Conjugative type IV secretion systems (T4SS) mediate bacterial conjugation, a process that enables the unidirectional exchange of genetic materials between a donor and a recipient bacterial cell. Bacterial conjugation is the primary means by which antibiotic resistance genes spread among bacterial populations. The recent cryo-electron microscopy (cryo-EM) structure of the conjugative Type 4 Secretion System (T4SS) encoded by the plasmid R388 revealed that the remaining VirB proteins form a large assembly organised into four sub-complexes: the outer membrane core complex (OMCC), the stalk, the arches and the inner membrane complex (IMC). Previously, we solved the cryo-electron microscopy (cryo-EM) structure of a conjugative T4SS. In this article, based on additional data, we present a more complete T4SS cryo-EM structure than that published earlier.

Also, a fourth subunit of TrwG/VirB8 in the asymmetric unit of both the Arches (TrwG/VirB8peri) and the IMC (TrwG/VirB8tail) could be placed and built. Correspondingly, a fourth TrwG/VirB8tail is observed in the asymmetric unit of the IMC. Therefore, overall, there are 24 TrwG/VirB8 subunits in the T4SS. An intriguing feature of the T4SS structure solved previously was the paucity of interactions between the various sub-complexes (OMCC, Arches, Stalk and IMC). However, from the work presented here, VirB10 emerges as a crucial and unique element that ‘glues’ these distinct sub-complexes together. Another remarkable feature of VirB10 is that the T4SS include 16 copies of them, only 14 are used in the O-layer, potentially only 12 of them in the Arches, with only five of those involved in VirB6 binding and six involved in VirB4 ATPase contacts. One of the two VirB10Arches that we have observed runs very close to the VirB2 assembly site on VirB6 and we now know that VirB10IM in the IM obstructs the VirB2 recruitment site on VirB6, providing two other means by which VirB10 may be regulating pilus subunit recruitment and assembly. Finally, we observe a sequence of VirB10 (VirB10Cyto) that makes multiple contacts with the TrwK/VirB4 ATPase, thereby potentially providing another point of pilus biogenesis regulation.

>MKKLVMTAAVAAILGAASPVMAQGIPVFDGTRALDFVQQFARMKEQLDTAKDQLAEAQRMYEAVTGGRGLGDLMRNAQLREYLPDDLRTVYDSANGGGYSGISGSINDILRDERLNGSVADMRRSIEERSRTAAATDKAVGLRAYEGAQQRLAQIEGLMDEISRTQDQKAIEELQARIAGEQAAIQNETTKLQMIAQLRQAEQALISEQRRERNMRILSSGNQGMPTIQ[5x];>MSKKQPKPVKAEQLKSYYEESRGLERDLIGEFVKSRKTAWRVATASGLFGLLGMVCGIVGFSQPAPAPLVLRVDNATGAVDVVTTLREHESSYGEVVDTYWLNQYVLNREAYDYNTIQMNYDTTALLSAPAVQQDYYKLFDGSNARDRVLGNKARITVRVRSIQPNGRGQATVRFTTQQHNSNGTVEAPQHQIATIGYTYIGAPMRSSDRLLNPLGFQVTSYRADPEILNN[12x];>[5x]MAFELFTPLFNKIDQTTATYVTDISSRAIAAITPVVSVGLTLGFITYGWLIIRGAVEMPVAEFLNRCLRIGIIVSIALAGGLYQGEIANAITTVPDELASALLGNPTQGASAAALVDQSAQQGFDRASEAFEEAGFFSSDGLLYGLFGIIILLATGLLAAIGGAFLLLAKIALALLAGLGPLFILALIWQPTHRFFDQWAQQVLNYGLLIVLFAAVFGLLMQIFGSYMADLRFDGAQNVAYAIGGSVILSIVSIVLLMQLPSIASGLAGGIGLGYMWELRSMRSGAGAAMRGGRAMARGARAAPGAARGAAVGAANMAKTVATGGAGVARAAAGYFRGRKAG;>MGAIESRKLLASETPVGQFIPYSHHVTDTIISTKNAEYLSVWKIDGRSHQSASEADVFQWIRELNNTLRGISSANLSLWTHIVRRRVYEYPDAEFDNVFCRQLDEKYRESFTGYNLMVNDLYLTVVYRPVSDKVLSFFAKRERETPDQKKHRQESCIKALEDINRTLGQSFKRYGAELLSVYEKGGHAFSAPLEFLARLVNGEHIPMPICRDRFSDYMAVNRPMFSKWGEVGELRSLTGLRRFGMLEIREYDDATEPGQLNVLLESDYEFVLTHSFSVLSRPAAKEYLQRHQKNLIDARDVATDQIEEIDEALNQLISGHFVMGEHHCTLTVYGETVQQVRDNLAHASAAMLDVAVLPKPVDLALEAGYWAQLPANWQWRPRPAPITSLNFLSFSPFHNFMSGKPTGNPWGPAVTILKTVSGTPLYFNFHASKEEEDATDKRLLGNTMLIGQSSSGKTVLLGFLLAQAQKFKPTIVAFDKDRGMEISIRAMGGRYLPLKTGEPSGFNPFQLPPTHANLIFLKQFVKKLAAAGGEVTHRDEEEIDQAITAMMSDSIDKSLRRLSLLLQFLPNPRSDDMDARPTVHARLVKWCEGGDYGWLFDNPTDALDLSTHQIYGFDITEFLDNPEARTPVMMYLLYRTESMIDGRRFMYVFDEFWKPLQDEYFEDLAKNKQKTIRKQNGIFVFATQEPSDALESNIAKTLIQQCATYIFLANPKADYEDYTQGFKLTDSEFELVRGLGEFSRRFLIKQGDQSALAEMNLGKFRTIVDGETVERDFDDELLVLSGTPDNAEIAESIIAEVGDDPAVWLPIFLDRVKAERSDV[6x];>MKPPQQQHEAFPLFKGATRLPTIWGVPMIPLMAMVMGVAVIALTVSIWWWALVPPLWFIMAQITKNDDKAFRIWWLWIDTKFRNRNKGFWGASSYSPANYRKRR[3x];>[3x]MFGRKKGDVIDAGAELERAEQERIEGEYGASELASERRPHTPGARTLLMVLLCVIAVVLVTLSYKAYKVRGVVEDDDAQPQQVVRQVIPGYTPRPIRPEPENVPEPPQPTTSVPAIQPAPVTQPVRPQPTGPREKTPYELARERMLRSGLTAGSGGGEDLPRPQGGDVPAGGLMGGGGGGGELAEKLQPMRLSGSSAGRLGNRDMLITQGTQLDCVLETRLVTTQPGMTTCHLTRDVYSTSGRVVLLDRGSKVVGFYQGGLRQGQARIFVQWSRIETPSGVVINLDSPGTGPLGEAGLGGWIDRHFWERFGGAIMISLIGDLGDWASRQGSRQGDNSIQFSNTANGVESAAAEALRNSINIPPTLYKNQGERVNILVARDLDFSDVYSLESIPTK The native ribonucleoprotein (RNP) particles are formed by the association of these single-stranded RNAs to multiple monomers of nucleoprotein (NP) and a single copy of the polymerase, a heterotrimer composed by the PB1, PB2 and PA subunits. Such RNPs are independent molecular machines responsible for transcription and replication of each virus gene. To better understand how these processes take place we have determined the three-dimensional structure of a model ribonucleoprotein particle that only contains 248 nucleotides of virus RNA but is biologically active in vitro and in vivo. The structure shows a circular appearance and includes 9 nucleoprotein monomers, two of which are associated to the polymerase complex.

The three-dimensional reconstruction obtained by imposing 9-fold symmetry lacked information about the polymerase complex but could achieve better resolution for the NP ring. We also carried out a docking of the atomic structure of the NP in the cryo-EM reconstruction. The handedness of the cryo-EM map was determined on the basis of the correlation coefficient of the NP atomic structure docked into the symmetrised volume. A good fit is observed between the two domains described in the atomic structure and the volume of the NP monomer. However, additional masses are observed at the top and at the bottom of each NP monomer. We propose that the extra mass at the top of the NP monomer corresponds to the protein sequences not solved in the crystal structure while that at the bottom may contain genomic RNA. The interaction among NP monomers is conserved in the NP docking presented here, with the only need to alter the angle between NP monomers from about 120° in the crystal to 40° in the RNP volume. This interaction interface would be more realistic, as no NP trimeric structure has been described in natural virus RNPs, and would imply a small change in the arrangement of the connections between the loop and the body of the NP (positions 428–438 and 396–402). The model obtained is compatible with the interaction mode proposed earlier and further indicated that additional side-by-side interactions are now possible due to the tighter packing of the monomers (black arrow). The relevance of the 420–428 loop in the NP-NP interaction was verified functionally: The contacts of amino acid R416 and F412 are essential for replication, while amino acid K422 does not appear to be important, in spite of being conserved among type A and B viruses.

>RSYEQMETDGERQNATEIRASVGKMIDGIGRFYIQMCTELKLSDYEGRLIQNSLTIERMVLSAFDERRNKYLEEHPSAGKDPKKTGGPIYRRVDGKWRRELILYDKEEIRRIWRQANNGDDATAGLTHMMIWHSNLNDATYQRTRALVRTGMDPRMCSLMQGSTLPRRSGAAGAAVKGVGTMVMELIRMIKRGINDRNFWRGENGRRTRIAYERMCNILKGKFQTAAQRTMVDQVRESRNPGNAEFEDLIFLARSALILRGSVAHKSCLPACVYGSAVASGYDFEREGYSLVGIDPFRLLQNSQVYSLIRPNENPAHKSQLVWMACHSAAFEDLRVSSFIRGTKVVPRGKLSTRGVQIASNENMETMESSTLELRSRYWAIRTRSGGNTNQQRASSGQISIQPTFSVQRNLPFDRPTIMAAFTGNTEGRTSDMRTEIIRLMESARPEDVSFQGRGVFELSDEKATSPIVPSFDMSNEGSYFFGDNAEEYDNLEHHHHHH[9x]>[2x]MKLHERLRELRSERGLRLKDVAEVAQISVPYLSDLERGRTNPSLETLQTLAGA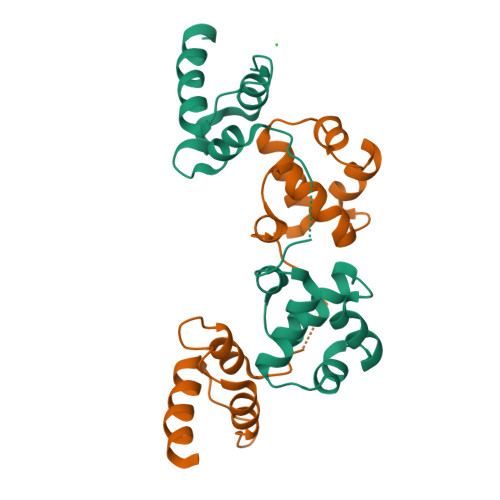YNITVHDLLEGVEFYGASTEGALPKGLSDLIADPTLGPQITPDWVRTLSRIELRGKRPRDKQDWYEIYLHLKRILS5'-(hydrazinecarbonyl)[2,2'-bipyridine]-5-carboxamide 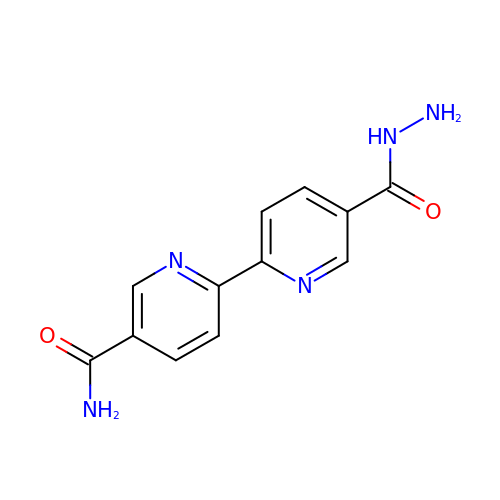| C12 H11 N5 O2 | HCFBUFHFZAJOFM-UHFFFAOYSA-N> GPLGSLTASMLASAPPQEQKQMLGERLFPLIQAMHPTLAGKITGMLLEIDNSELLHMLESPESLRSKVDEAVA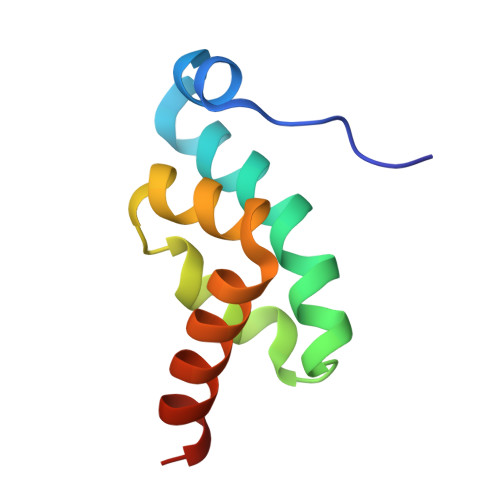VLQAHQA> ASLTEIEHLVQSVC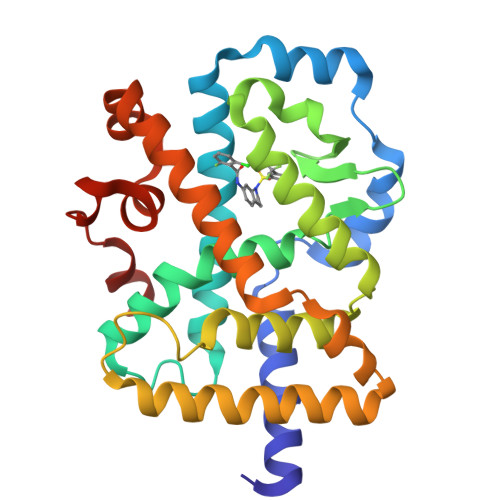KSYRETCQLRLEDLLRQRSNIFSREEVTGYQRKSMWEMWERCAHHLTEAIQYVVEFAKRLSGFMELCQNDQIVLLKAGAMEVVLVRMCRAYNADNRTVFFEGKYGGMELFRALGCSELISSIFDFSHSLSALHFSEDEIALYTALVLINAHRPGLQEKRKVEQLQYNLELAFHHHLCKTHRQSILAKLPPKGKLRSLCSQHVERLQIFQHLHPIVVQAAFPPLYKELFSGGGEKHKILHRLLQDS> GGCCGACGGAGGCGCGCCCGAGAUGAGUAGGCUGUCCCAUCAGGGGAGGAAUCGGGGACGGCUGAAAGGCGAGGGCGCCGAAGGGUGCAGAGUUCCUCCCGCUCUGCAUGCCUGGGGGUAUGGGGAAUACCCAU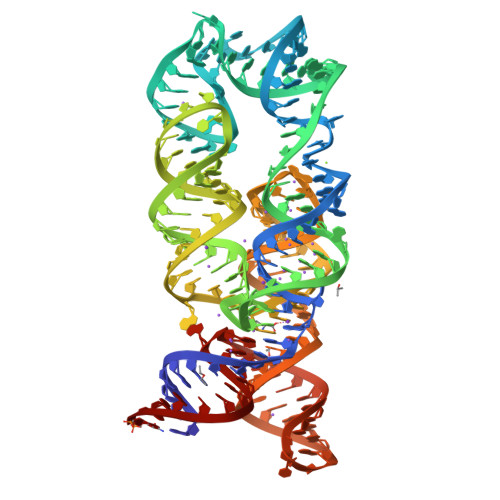ACCACUGUCACGGAGGUCUCUCCGUGGAGAGCCGUCGGUC>GPLGSPEFIILQTYRAIADYEKTSGSEMALSTGDVVEVVEKSESGWWFCQMKAKRGWIPASFLEPLDSPDETEDPEPNYAGEPYVAIKAYTAVE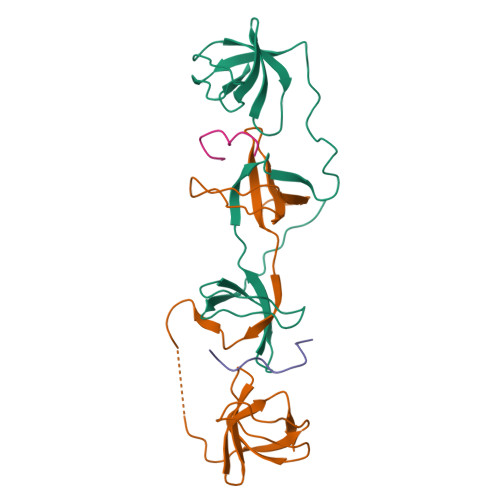GDEVSLLEGEAVEVIHKLLDGWWVIRKDDVTGYFPSMYLQKSGQ[2x];>[2x]KQPPSNPPPRPPAEARKK> MAAGPISERNQDATVYVGGLDEKVSEPLLWELFLQAGPVVNTHMPKDRVTGQHQGYG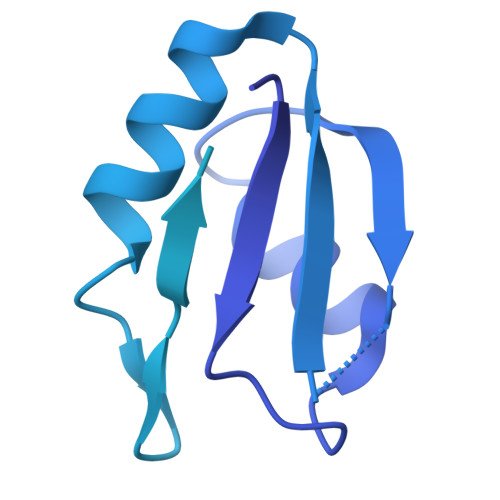FVEFLSEEDADYAIKIMNMIKLYGKPIRVNKASAHNKNLDVGANIFIGNLDPEIDEKLLYDTFSAFGVILQTPKIMRDPDTGNSKGYAFINFASFDASDAAIEAMNGQYLCNRPITVSYAFKKDSKGERHGSAAERLLAAQNPLSQADRPHQLFADAPPPPSAPNPVVSSLGSGLPPPGMPPPGSFPPPVPPPGALPPGIPPAMPPPPMPPGAAGHGPPSAGTPGAGHPGHGHSHPHPFPPGGMPHPGMSQMQLAHHGPHGLGHPHAGPPGSGGQPPPRPPPGMPHPGPPPMGMPPRGPPFGSPMGHPGPMPPHGMRGPPPLMPPHGYTGPPRPPPYGYQRGPLPPPRPTPRPPVPPRGPLRGPLPQ> MSVGLIAPLASPIQESRANTNIENIGDGAEVIKRTEDVSSKKWGVTQNVQFDFVKDKKYNKDALIVKMQGFINSRTSFSDVKGSGYELTKRMIWPFQYNIGLTTKDPNVSLINYLPKNKIETTDVGQTLGYNIGGNFQSAPSIGGNGSFNYSKTISYTQKSYVSEVDKQNSKSVKWGVKANEFVTPDGKKSAHDRYLFVQSPNGPTGSAREYFAPDNQLPPLVQSGFNPSFITTLSHEKGSSDTSEFEISYGRNLDITYATLFPRTGIYAERKHNAFVNRNFVVRYEVNWKTHEIKVKGHNKHHHHHH

Staphylococcus aureus (SA) leukocidin ED (LukED) belongs to a family of bicomponent pore forming toxins that play important roles in SA immune evasion and nutrient acquisition. LukED targets specific G protein-coupled chemokine receptors to lyse human erythrocytes (red blood cells) and leukocytes (white blood cells). Each leukotoxin is made up of two subunits of approximately 30 kDa: a host cell targeting S-component (HlgA, HlgC, LukE, lukS-PV, and LukA/G), and a polymerization F- component (HlgB, LukD, lukF-PV, and LukB/H), which can bind the plasma membrane through highly conserved phosphocholine binding sites. Each toxin is composed of two domains: a central β sandwich called the CAP domain and involved in inter-protomer interactions, and a RIM domain which contains several divergent loops driving host cell specificity.

While attempting to co-crystallize LukE in complex with peptides encompassing the sulfated ACKR1 Tyr41 residue, we serendipitously obtained two additional apo crystal forms of LukE at 1.5 Å (apo1) and 1.9 Å (apo2), allowing us to build a higher quality model. Rg values of the selected models were in a narrow range between 2.40 and 2.55 nm, consistent with the values of 2.32 and 2.43 nm calculated from the apo1 and apo2 structures.>MTASHGQAAAIPTVTLNDDNTLPVVGIGVGELSDSEAERSVSAALEAGYRLIDTAAAYGNEAAVGRAIAASGIPRDEIYVTTKLATPDQGFTSSQAAARASLERLGLDYVDLYLIHWPG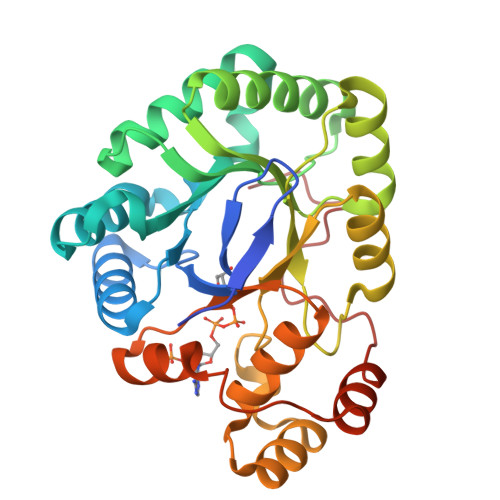GDTSKYVDSWGGLMKVKEDGIARSIGVCNFGAEDLETIVSLTYFTPAVNQIELHPLLNQAALREVNAGYNIVTEAYGPLGVGRLLDHPAVTAIAEAHGRTAAQVLLRWSIQLGNVVISRSANPERIASNLDVFGFELTADEMETLNGLDDGTRFRPDPATYTGS[2x]>GAASSDYVIDDKVAILQKRDHEGFGFVLRGAKAETPIEEFTPTPAFPALQYLESVDVEGVAWRAGLRTGDFLIEVNGVNVVKVG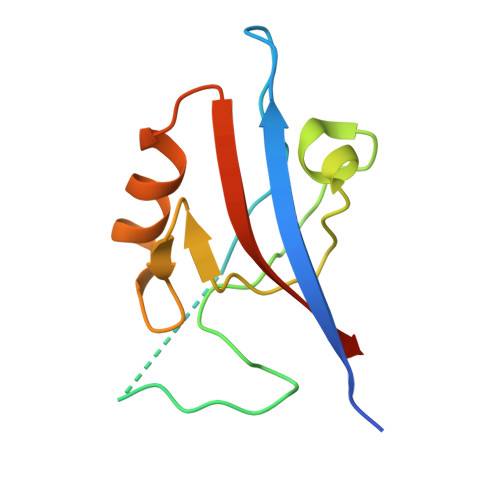HKQVVGLIRQGGNRLVMKVVSVTRKPEE[8x]>GPAVKRLLGWKQGDEEEKWCEKA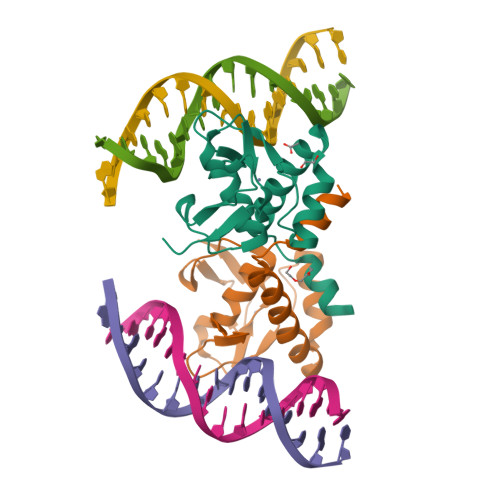VKSLVKKLKKTGQLDELEKAITTQNVNTKCITIPRSLDGRLQVSHRKGLPHVIYCRLWRWPDLHSHHELRAMELCEFAFNMKKDEVCVNPYHYQRVETPVLP[2x]>GPVPHFAEADIVTLQGVTGGNTFAVPALPPGAVGDGPPRVDFPRSRLRFKEKLGEGQFGEVHLCEVDSPQDLVSLDFPLNVRKGHPLLVAVKILRPDATKNARNDFLKEVKIMSRLKDPNIIRLLGVCVQDDPLCMITDYMENGDLNQFLSAHQLEDKAAEGAPGDGQAAQGPTISYPMLLHVAAQIASGMRYLATLNFVHRDLATRNCLVGENFTIKIADFGMSRNLYAGDYYRVQGRAVLPIRWMAWECILMGKFTTASDVWAFGVTLWEVLMLCRAQPFGQLTDEQVIENAGEFFRDQGRQVYLSRPPACPQGLYELMLRCWSRESEQRPPFSQLHRFLAE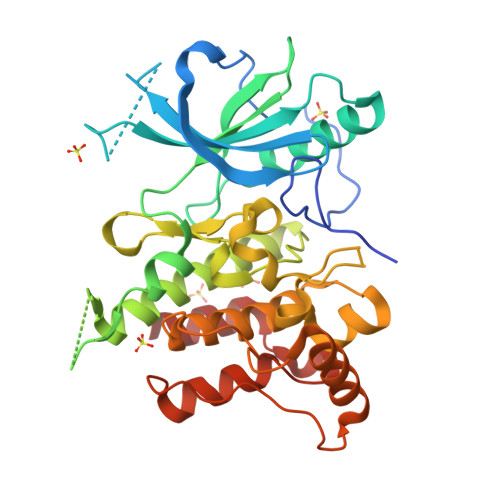DALNTV[3x]>[2x]GMEFYEVIKKRKSIKKFEQTAIDRDKLLKIIDMAMRAPSWKNKTPYKFIVVESDKLKLDIANAIENKTSAASEAVLNSPMT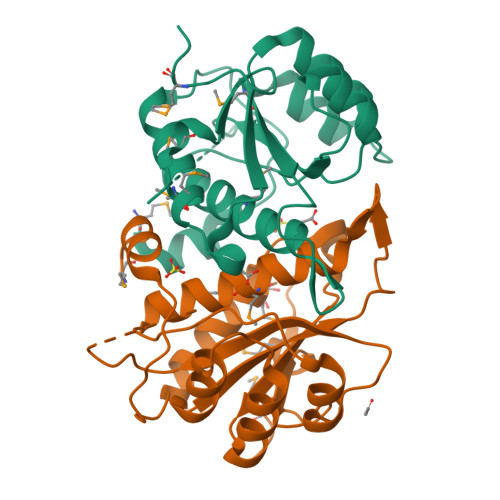IVAVANPEESGDVSGKEIYLIDTAIAMEHIVLGATDEGYGTCWIAAFNENKIKEALKIPDNLRVVALTPLGVPKDSAEDEPHHPKKDMDEYLYIDKWGTSFMESNVKILEKN> MANEEDDPVVQEIDVYLAKSLAEKLYLFQYPVRPASMTYDDIPHLSAKIKPKQQKVELEMAIDTLNPNYCRSKGEQIALNVDGACADETSTYSSKLMDKQTFCSSQTTSNTSRYAAALYRQGELHLTPLHGILQLRPSFSYLDKADAKHREREAANEAGDSSQDEAEDDVKQITVRFSRPESEQARQRRVQSYEFLQKKHAEEPWVHLHYYGLRDSRSEHERQYLLCPGSSGVENTELVKSPSEYLMMLMPPSQEEEKDKPVAPSNVLSMAQLRTLPLADQIKILMKNVKVMPF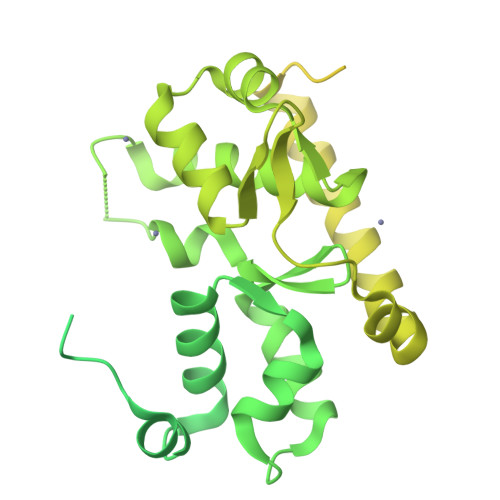ANLMSLLGPSIDSVAVLRGIQKVAMLVQGNWVVKSDILYPKDSSSPHSGVPAEVLCRGRDFVMWKFTQSRWVVRKEVATVTKLCAEDVKDFLEHMAVVRINKGWEFILPYDGEFIKKHPDVVQRQHMLWTGIQAKLEKVYNLVKETMPKKPDAQSGPAGLVCGDQRIQVAKTKAQQNHALLERELQRRKEQLRVPAVPPGVRIKEEPVSEEGEEDEEQEAEEEPMDTSPSGLHSKLANGLPLGRAAGTDSFNGHPPQGCASTPVARELKAFVEATFQRQFVLTLSELKRLFNLHLASLPPGHTLFSGISDRMLQDTVLAAGCKQILVPFPPQTAASPDEQKVFALWESGDMSDQHRQVLLEIFSKNYRVRRNMIQSRLTQECGEDLSKQEVDKVLKDCCVSYGGMWYLKGTVQS> DMACHKIPVDADFLYAYSTAPGYYSWRNSKDGSWFIQSLCAMLKQYADKLEFMHILTRVNRKVATEFESFSFDATFHAKKQIPC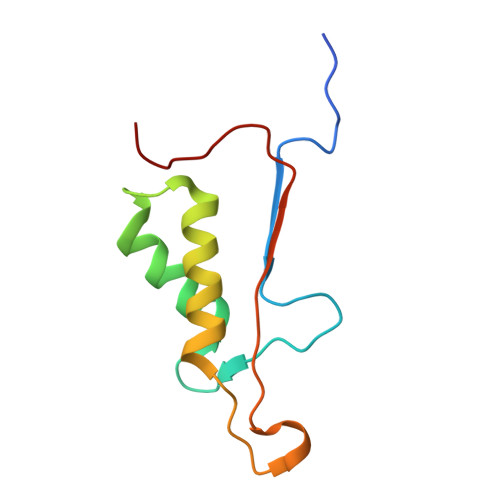IVSMLTKELYFYH> AASGSALIFDEEMSRYKLLWTDPACEIEVPERLTVSYEALRTHGLAQRCKAVPVRQATEQEILLAHSEEYLEAVKQTPGMNVEELMAFSKKYNDVYFHQNIYHCAKLAAGATLQLVDSVMKREVRNGMALVRPPGHHSQRSAANGFCVFNNVAFAALYAKKNYNLNRILIVDWDVHHGQGIQYCFEEDPSVLYFSWHRYEHQSFWPNLPESDYSSVGKGKGSGFNINLPWNKVGMTNSDYLAAFFHVLLPVAYEFDPELVIVSAGFDSAIGDPEGEMCALPEIFAHLTHLLMPLAAGKMCVVLEGGYNLTSLGQSVCQTVHSLLGDPTPRISGLGTACDSALESIQNVRNVQSSYWSSFKHLAQSETNPKRPRLDATNGGPKESSEPASESNPKKTAQDIVWPEPLK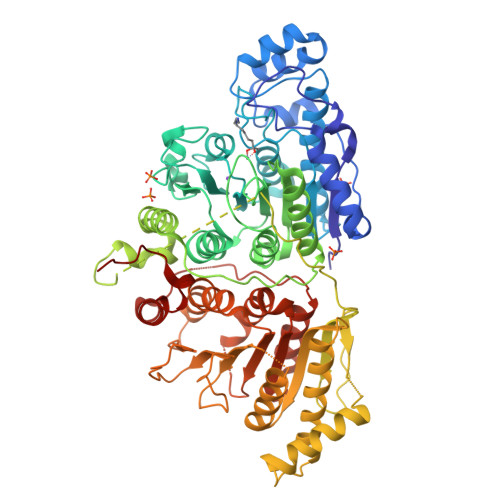RMPASVRTVVVPPPGVELTLPKNCQHSGDISESTAKEVQRIRDKHFHDLTDQNILRSLGNIISVLDRMMRSDEVCNGCVVVSDLSVSVQCALQHALTEPAERVLVVYVGDGELPVKTNDGKVFLVQICTKETEDKCVNRLTLCLREGESLTAGFMQALLGLILPVAYEFNPALVLGIVEETAAKTRLMRVWGHMTCLIQGLARGRMLTLLQGYDKDLLELTVSALSGASISPLGPLRAPKPEDVEMMEKQRQRLQERWGLLRCTVSESW> MTLSLANYLAADSAAEALRRDVRAGLTAAPKSLPPKWFYDAVGSDLFDQITRLPEYYPTRTEAQILRTRSAEIIAAAGADTLVELGSGTSEKTR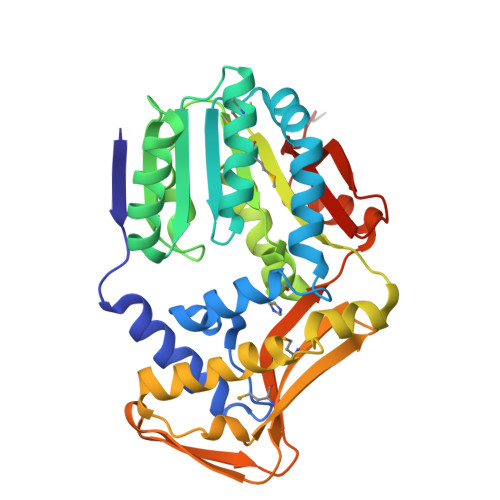MLLDAMRDAELLRRFIPFDVDAGVLRSAGAAIGAEYPGIEIDAVCGDFEEHLGKIPHVGRRLVVFLGSTIGNLTPAPRAEFLSTLADTLQPGDSLLLGTDLVKDTGRLVRAYDDAAGVTAAFNRNVLAVVNRELSADFDLDAFEHVAKWNSDEERIEMWLRARTAQHVRVAALDLEVDFAAGEEMLTEVSCKFRPENVVAELAEAGLRQTHWWTDPAGDFGLSLAVRLEHHHHHH>[2x]MTSATASFATRTSLAADLAALGLAWGDAIMVHAAVSRVGRLLDGPDTIIAALRDTVGPGGTVLAYADWEARYEDLVD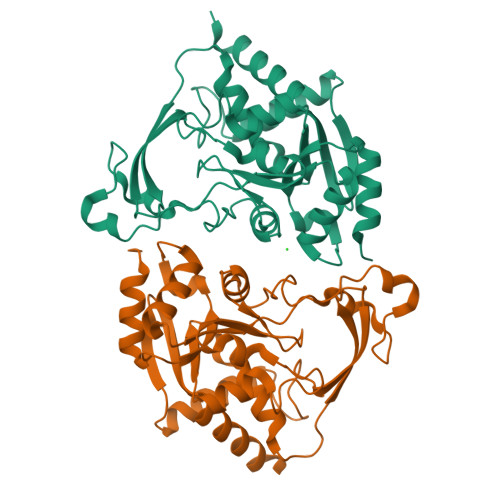DAGRVPPEWREHVPPFDPQRSRAIRDNGVLPEFLRTTPGTLRSGNPGASLVALGAKAEWFTADHPLDYGYGEGSPLAKLVEAGGKVLMLGAPLDTLTLLHHAEHLADIPGKRIKRIEVPFATPTGTQWRMIEEFDTGDPIVAGLAEDYFAGIVTEFLASGQGRQGLIGAAPSVLVDAAAITAFGVTWLEKRFGTPSP Cyclic β-1,2-glucan (CβG) is a circular polysaccharide critical for host interactions of many bacteria, including major pathogens of humans (Brucella) and plants (Agrobacterium). The production of the main CβG chain occurs in the cytoplasm and is orchestrated by the cyclic glucan synthase (Cgs), a large, multi-domain membrane protein that contains several enzymatic sites. We determine the structure of this complex protein machinery and clarify key aspects of CβG synthesis, revealing a distinct mechanism that uses a tyrosine-linked oligosaccharide intermediate in cycles of polymerization and processing of the glucan chain.

In order to determine the structure of Cgs, we constructed a strain of A. tumefaciens C58 carrying an insertion in the chromosomal copy of the chvB gene encoding a C-terminal 3xFlag-tag (CgsWT). The CgsWT and CgsiGP samples produced high resolution maps of the full-length protein. The CgsWT map contains a disordered density docked at the active site of CY, which could potentially correspond to a glucan chain reaction intermediate. The CgsWT and CgsiGP3 maps obtained in the presence of UDP-Glc contain additional densities of glucan chain fragments bound to the protein at the cytoplasmic side of the CTD. This surface, which stretches between the CY and GP enzymatic pockets, appears to contain affinity sites capable of coordinating the polysaccharide. The first site, at the CY active site (CgsWT map), contains a disordered density. We found that an additional mass corresponding to 9- and 3-glucose chains is attached to the IF1-homology loop in CgsWT, while no such modifications were detected in CgsiGT.

> MSFHITPTAAARDSETKQIDHNDSIRASYMTIEELHDAGAALSRDGADSLPGFMEFDFFERHRENEKEILRVYRTTAVDAENGATITPAAEWLLDNHYVIEEAIQEVRRDFPRKFYRQLPTMTVGGVTIPRVMALGWLYVAHTHSTVSRENMTALVDGYQTSQTLQIGELWALPSIIRFVLIENLRRISIRVERSRRMRQKANEVVDEIIRLNDAEASAALLKQVDSLVDDPTFATQFLYRLRNGSQTSGFAVAWLEERLHAAGTDAENVMMSEHNRLASGNVTMGNIVKSLREIDDTEWSVWFEEVSHIDKVLREETDYEILDFGSRNTYRNTIELLARRSPRTEVEVARAAVEMARSDLPAGADENHRVNVGSVLVGQRRFELEKALGYRPLASQHIVRSMRKFNWLAIAAPVLLITAVAMLAVGWFLAKAGMPWYVVTAFLLMFALPASEGATGLFNTLVTFFVKPFRLVGYEFKNGIPEDARTLVAVPCMLTSRDSVDEMMRNIEVHYLANPHGEIYFSLVSDWRDAPYEQSDEDLEILDYAKRELAALNSRYAFDGKTRFYLLHRRRIYNSAEECWMGWERKRGKLHELNMLLRGDKDTTFLGGSNIVPADVKYVMTLDADTRLMRDAVTKLVGKMHHPINRPKIDPVSGRVVEGYGLLQPRVTPSLTTGKDASVFQRVFSINRGIDPYVFTVSDVYQDLTSEGTFTGKGLYDVDAFEAALKGRIEENSILSHDLLEGSFARCALVTDVELVEDFPTRYEVEVSRQHRWARGDWQLLPFIIDRARGVTAIGRWKMVDNLRRSLTPIAWFFASILGWYFMDPLGALIWQILLIFSLFVAPTLSLLSGLVPRSTDIVPQAHFFTIWSEIRATNAQVALRIVFIADAACMMTDAIVRSLYRLLVSHKLMLEWRTAASMQSSAQGSIVDYYRQMWHAPVVAMLGLLFAALPGDNAFLIGIPFTLLWVLSPAVAWYVSQSAETEDRLFVSEHVSFELRKIARRTWRYYEAFVTPQENHLPPDNFQETPEPIVASRTSPTNIGVYLLSVISARQFGWISFADTLERIENTIQTVEKMEKHRGHLYNWYHTDTLQTLGPRYVSAVDSGNLAGHLIAVSSACRDWAEAPSAHLQGNLDGIGDVAGILRETLKALPDNRKTLRPLHRRLEERIIGFSNALASVKREHEFASIRVINLAVLARDIQKLATNVDHEVKSAQSAEVTRWAQLLVESCEAHISDSAIDLTNMEPLRQRLASLRDRSRNLAFSMDFTFLYRKDRRLLSIGYRVESKELDEACYDLLASECRLTSLFAIAKGDLPTEHWYRLGRQVVPIGAQGALVSWSGSMFEYLMPPLVMQERQGGILNQTNNLIVKEQMNHGRRLGTPWGISEAAFNARDHNMNYQYTNFGVPTLGLKRGLGQNAVIAPYASILASQYDPDGALENLDKLRKLGALGQYGFHDAVDFTPTRVPDGKVCAVVYNYYAHHHGMSIAAVANVAFDGVLRELFHSDPVIEAAELLLQEKAPREVPVMSAKYEPETPGKEQADLLRAEVRSIADPAVRDREVVFLSNGHYSTMLTSTGAGYSKWNGQAISRWKADPTDDRWGTFIFLRDTTNGQWWSATAEPRVIEGEKTKTIFTDDKAEFHKTIGDLQSVVECIVATEHDAEGRRITLLNVGSEDRYIEVTSYMEPVIASEDDDNAHPLFSRMFVQTEIGRRGDVIRAWRNRRSQNEPGTVIAHLAADNAGPSRPTEFETDRAKFIGRGRSLREAAAFDAGATLSSSDGFTLDPILSLRRTVRVPAGKKVSVIFWTIAAPSREEVDKAIDRYRHPDAFAHELVHAWTRTQVQMRHVGVTSQQAAAFQHLGRYLTYPDMHLRADSETLKTGLASQRALWPLAISGDFPIFSLRINDDMDMDIAREALSAHEYLRSRGVIFDLVIVNERAASYAQDMQHALDHISETQRRINPADGGRPHVFSVRRDLMDEETWSALLAASRVVLHVRNGKIVDQINRAVSLFAANRGPDGSSDAAQARLPVPAFPVAEPVEDAGDLDFWNGFGGFAKNGQEYVVRLNGGQSTPHPWINVISNENFGFHISAEGAGFSWSRNSRDYQLTPWTNDPVINRPGEAFYVADVETGKLYTPCAALSRDPEAMFETRHGLGYSILTGVADTLEVELTQTVDREKPVKFSQVIVRNKGSKSRRLKVYAYVEWVLGNNGQKSAPFILSRHDAGSNAIFASNPYSIDYSARTSFLTLDSEASGFTTSRREFIGRFGSAQAPQGIVAGAALSGTTEVDGDPCAALMQEIHLKPGEERHMTFILGDADNAEEAEALVKDVRQADFLSVLEESKKFWTGFTGQLQVSTPDAGFNHMVNNWLPYQALACRILARTAFYQSSGAFGFRDQLQDTLAFLLYQPDLARTQILRAAGRQFPEGDVQHWWLPLTGAGVRTTISDDVVWLAYAINQYVSATGDAAILDESIPFLKGPALMPGQHDAFFQPETSERSATLYEHAALALDLAIHRTGENGLPLILGGDWNDGMNRVGVGGKGTSVWLGWFLAGALRDFIEIAEKRGDTDRVGKWASHREKLRHVLETAGWDGSYYRRGYFDDGTPLGSASSEECQIDSLGQSWSVLSGEGEEGRSRQAMDAVMEHLVDEKTGIIRLFTPPFSRASHDPGYIKGYPPGVRENGGQYTHAATWVVLALAKQGRAQEAWNCFKLLNPVNHALDAASSETYRVEPYVVTADVYGEGAYAGRGGWSWYTGSAGWLYRAAVEGILGITRTDGKLHVSPSLPEDWSGFSIRITLDGKARDIAVSRKAGTADVSVSVDG> GHMAQSETVERILDAAEQLFAEKGFAETSLRLITSKAGVNLAAVNYHFGSKKALIQAVFSRFLGPFCASLEKELDRRQAKPEAQHATLEDLLHLLVSQAMAVKPRSGNDLSIFMRLLGLAFSQSQGHLRKYLEEVYGKVFRRYMLLVNEAAPKLPPIELFWRVHFMLGAAAFSMSGIKALRAMAETDFGVNTSTEQVMHLMVPFFAAGMRAESGI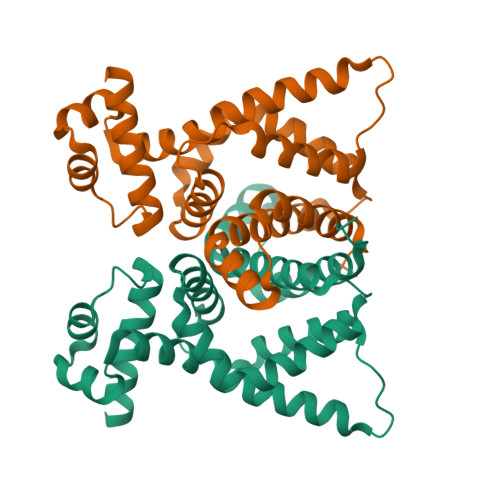DDPLLAGAQLRPRNKTPAKA>NAPVDLTPYILPGVSFLSDIPQETLSEIRNQTIRGEAQIRLGELMVSIRPMQVNGYFMGSLNQDGLSNDNIQIGLQYIEHIERTLNHGSLTSREVTVLREIEMLENMDLLSNYQLEELLDKIEVCAFNVEHAQLQVPESLRTCPVTLCEPEDGVFMR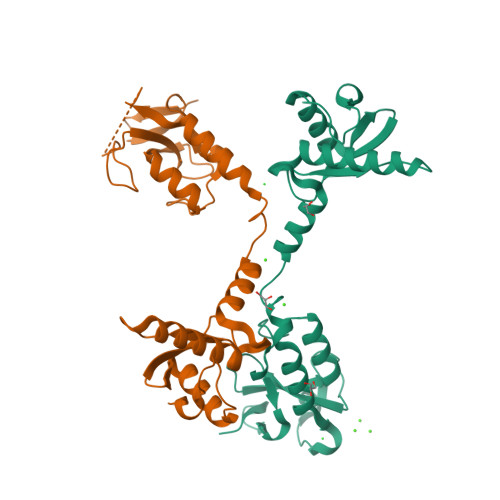NSMNSNVCMLYDKMALIHLVKTRAAHPLSRESIAVSMIVGRDNAAFDPDRGNFVLKN[2x]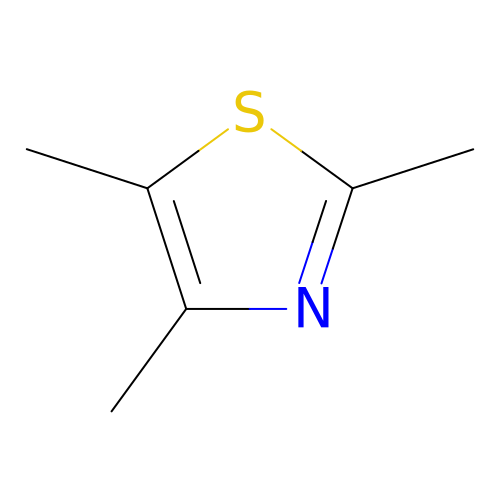2,4,5-trimethyl-1,3-thiazole | C6 H9 N S | BAMPVSWRQZNDQC-UHFFFAOYSA-N>[3x]MSKLASPQSVRALLERHGLFADKRFGQNFLVSEAHLRRIVEAARPFTGPVFEVGPGLGALTRALLEAGAEVTAIEKDLRLRPVLEETLSGLPVRLVFQDALLYPWEEVPQGS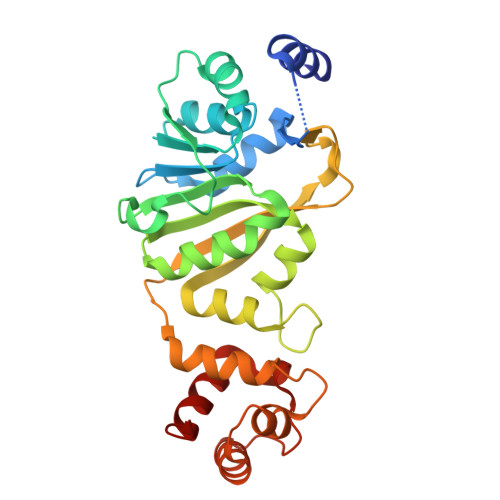LLVANLPYHIATPLVTRLLKTGRFARLVFLVQKEVAERMTARPKTPAYGVLTLRVAHHAVAERLFDLPPGAFFPPPKVWSSLVRLTPTGALDDPGLFRLVEAAFGKRRKTLLNALAAAGYPKARVEEALRALGLPPRVRAEELDLEAFRRLREGLEGAV> MAGFWVGTAPLVAAGRRGRWPPQQLMLSAALRTLKHVLYYSRQCLMVSRNLGSVGYDPNEKTFDKILVANRGEIACRVIRTCKKMGIKTVAIHSDVDASSVHVKMADEAVCVGPAPTSKSYLNMDAIMEAIKKTRAQAVHPGYGFLSENKEFARCLAAEDVVFIGPDTHAIQAMGDKIESKLLAKKAEVNTIPGFDGVVKDAEEAV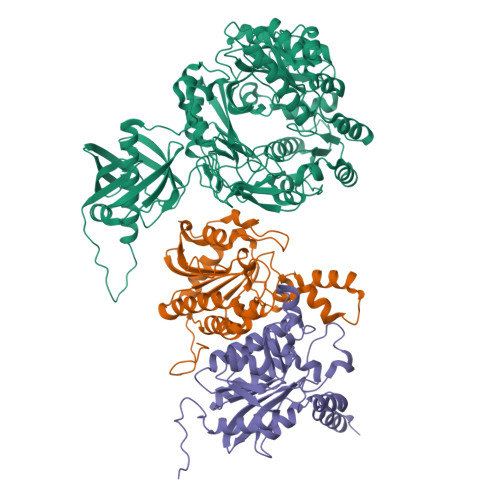RIAREIGYPVMIKASAGGGGKGMRIAWDDEETRDGFRLSSQEAASSFGDDRLLIEKFIDNPRHIEIQVLGDKHGNALWLNERECSIQRRNQKVVEEAPSIFLDAETRRAMGEQAVALARAVKYSSAGTVEFLVDSKKNFYFLEMNTRLQVEHPVTECITGLDLVQEMIRVAKGYPLRHKQADIRINGWAVECRVYAEDPYKSFGLPSIGRLSQYQEPLHLPGVRVDSGIQPGSDISIYYDPMISKLITYGSDRTEALKRMADALDNYVIRGVTHNIALLREVIINSRFVKGDISTKFLSDVYPDGFKGHMLTKSEKNQLLAIASSLFVAFQLRAQHFQENSRMPVIKPDIANWELSVKLHDKVHTVVASNNGSVFSVEVDGSKLNVTSTWNLASPLLSVSVDGTQRTVQCLSREAGGNMSIQFLGTVYKVNILTRLAAELNKFMLEKVTEDTSSVLRSPMPGVVVAVSVKPGDAVAEGQEICVIEAMKMQNSMTAGKTGTVKSVHCQAGDTVGEGDLLVELE;> DPSDRLVPELDTIVPLESTKAYNMVDIIHSVVDEREFFEIMPNYAKNIIVGFARMNGRTVGIVGNQPKVASGCLDINSSVKGARFVRFCDAFNIPLITFVDVPGFLPGTAQEYGGIIRHGAKLLYAFAEATVPKVTVITRKAYGGAYYVMSSKHLCGDTNYAWPTAEIAVMGAKGAVEIIFKGHENVEAAQAEYIEKFANPFPAAVRGFVDDIIQPSSTRARICCDLDVLASKKVQRPWRKHANIPL;> MAAALRVAAVGARLSVLASGLRAAVRSLCSQATSVNERIENKRRTALLGGGQRRIDAQHKRGKLTARERISLLLDPGSFVESDMFVEHRCADFGMAADKNKFPGDSVVTGRGRINGRLVYVFSQDFTVFGGSLSGAHAQKICKIMDQAITVGAPVIGLNDSGGARIQEGVESLAGYADIFLRNVTASGVIPQISLIMGPCAGGAVYSPALTDFTFMVKDTSYLFITGPDVVKSVTNEDVTQEELGGAKTHTTMSGVAHRAFENDVDALCNLRDFFNYLPLSSQDPAPVRECH>[2x]GAMGSGMAMDTFITRNFQTTIIQKAKNTMAEFSEDPELQPAMLFNTCVHLEVCYVISDMNFLDEEGKSYTALEGQGKEQNLRPQYEVIEGMPRTIAWMVQRSLAQEHGIETPKYLADLFDYKTKRFIEVGITKGLADDYFWKKKEKLGNSMELMIFSYNQDYSLSNESSLDEEGKGRVLSRLTELQAELSLKNLWQVLIGEEDVE

The heterotrimeric RNA-dependent RNA polymerase (RdRp) of influenza virus is composed of subunits PA, PB1 and PB2. It is responsible for replication and transcription of the segmented, single-stranded viral RNA genome (vRNA) in the nucleus of infected cells. Transcription of viral mRNAs occurs through a unique “cap-snatching” mechanism. We initially screened metal-chelating compounds by CEN enzymatic assays, followed by a cellular phenotypic screen and then optimized the chemical structure to improve the pharmacokinetics and safety. This culminated in the generation of the compounds BXA and BXM that target the CEN in the PA proteins of influenza A and B viruses.

In addition, a structure of the influenza B domain with the I38T mutation was determined without bound compound at 1.8 Å resolution. For the FluB I38T mutant in the absence of ligand, the threonine side-chain changes rotamer. The methyl-group is now in the position of the CG2 of the isoleucine and the hydroxyl group is only able to make one hydrogen bond with the carbonyl oxygen of Met34. Furthermore, in the unbound form, Met34 is orientated into the pocket and also has to change rotamer to accommodate the ligand in which case it packs against the heterocyclic fluorines of the tail-group. The results show a 10-fold reduced activity of the I38T mutant endonuclease in vitro for both FluA and FluB (black triangles). That Met34 is also important for substrate RNA binding could explain why, in the case of FluB, the I38T mutation has little impact on viral fitness.>MRFTILSVLAFSLPLVLAETPAPSCPVTNVTTPQLDPITQAYADAISSRPSLFAFPLPEIRDGYQSNVSDPSTEFTTKILSLPVGPTGNVTAYLYKPVSGEREKGKDLLPVIAYFHGGGWVFGGPKSYRGLITNLIRESGAAVFFVDYTLTPKVAYPVPNEQCYAAVQWLLEHGEKLGVDPTNMGFGGDSAGGELSSSVSLLSIKRKTPLPKFQVLIYPATDLACESATFKEFPNGPGLTTDEIRFAASLFTPDPKSRLEDVASPGRASDEDLAKFPETLIVVAEVDPIRQQGEDFGRRLQKLGVRAAIIRVLGTIHGFASIDVLSE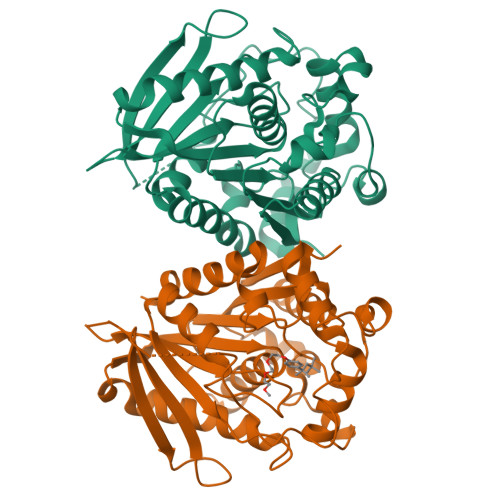APGAKATIELIGYKFKKALH[4x]>[2x]MFEQRVNSDVLTVSTVNSQDQVTQKPLRDSVKQALKNYFAQLNGQDVNDLYELVL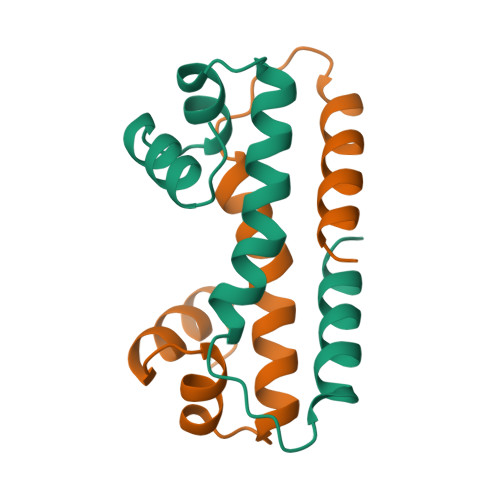AEVEQPLLDMVMQYTRGNQTRAALMMGINRGTLCKKLKKYGMN oxidanylphosphinate | H2 O3 P | 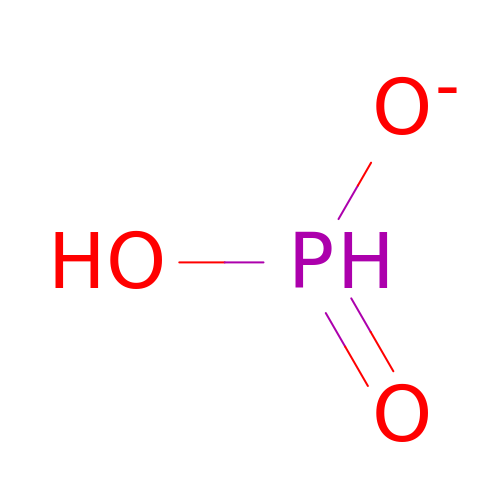ABLZXFCXXLZCGV-UHFFFAOYSA-M> VFPHPIYDYQDTEYLAKITIGAPGQSFHVVLDTGSANLWI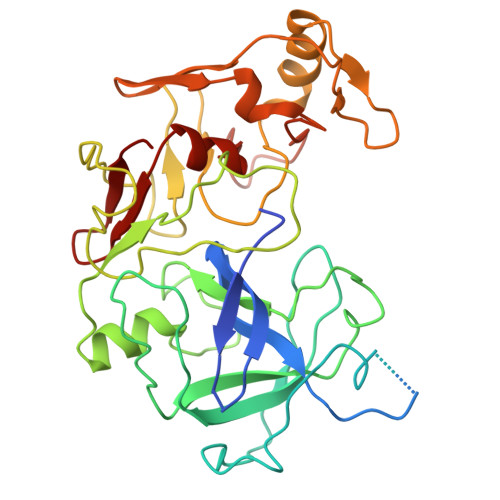PDNICVNGRRGACRITTCDRGLVCEVLCHDKSCCEDDVDNPDEDNPCKGKSGFDSTQSTSYAKITPKKYFEIVYGTGFAKGFLGNDTVRFGEEGNNKTLVVPGTVFGQAVQIGDPFANNPINGILGLGFRGLAQAGVTPPLQRAIDLKLVDPIFTVYMKQLGAKAKGQDGGAFTYGGLDSVNCGQEIAYVDLTRPLYWQFKMEAFSAGYLSIRKGWEVISDTGTSFMGVPTAIADLVADSYGGQYDEMFEIYTVDCNATVTFGMTIGGKQYKIERKNLVLEEDKDSCMIAMTPLSSVGFGPQWILGAPFIRQYCNIHDMRNNTIGFAEP>[2x]MGMWASLDALWEMPAEKRIFGAVLLFSWTVYLWETFLAQRQRRIYKTTTHVPPELGQIMDSETFEKSRLYQLDKSTFSFWSGLYSETEGTLILLFGGIPYLWRLSGRFC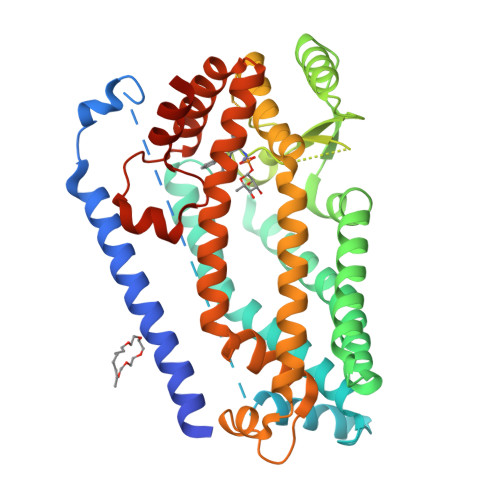GYAGFGPEYEITQSLVFLLLATLFSALAGLPWSLYNTFVIEEKHGFNQQTLGFFMKDAIKKFVVTQCILLPVSSLLLYIIKIGGDYFFIYAWLFTLVVSLVLVTIYADYIAPLFDKFTPLPEGKLKEEIEVMAKSIDFPLTKVYVVEGSKRSSHSNAYFYGFFKNKRIVLFDTLLEEYSVLNKDIQEDSGMEPRNEEEGNSEEIKAKVKNKKQGCKNEEVLAVLGHELGHWKLGHTVKNIIISQMNSFLCFFLFAVLIGRKELFAAFGFYDSQPTLIGLLIIFQFIFSPYNEVLSFCLTVLSRRFEFQADAFAKKLGKAKDLYSALIKLNKDNLGFPVSDWLFSMWHYSHPPLLERLQALKTMKQHSGLEVLFQ5-(3-aminophenyl)furan-2-carboxamido-(beta-L-fucopyranose) | C17 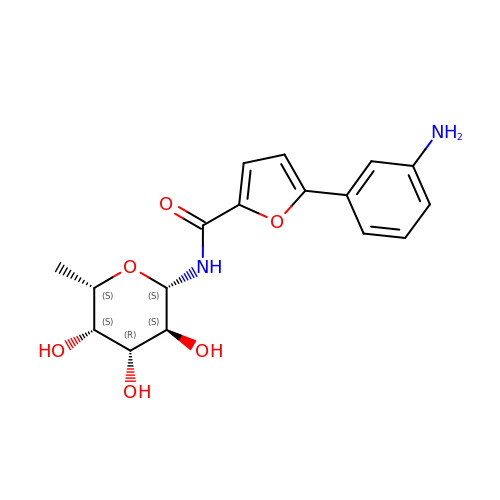H20 N2 O6 | QWRWVIPPQRQFMW-VUBKLASDSA-N>SNAMIPAKLKQGDEIRIIAPSRSIGIMADNQVEIAVNRLTDMGFK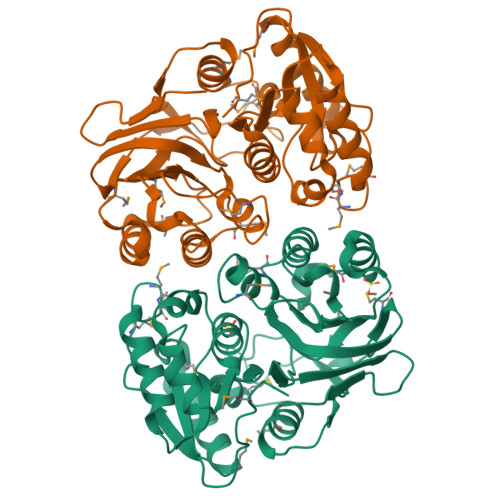VTFGEHVAEMDCMMSSSIRSRVADIHEAFNDSSVKAILTVIGGFNSNQLLPYLDYDLISENPKILCGFSDITALATAIYTQTELITYSGAHFSSFSMEKGLDYVMESFSDCLLQKEPFALKESATWSDDEWYLDQENRNFIPNEGLVVMQPGVAEGIIIGGNLCTLNLLQGTEYMPNLAGTILFIEDDFMTIPETFDRDLESLLSQPGADEIEGMVIGRFQQKTAMTAEKLAYIIETKTALQKIPVISGADFGHTQPIATFPIGGTARIDTNQTDKIQIIRH[2x]In Gram-negative bacteria, Fe3+-siderophore complexes are recognised at the bacterial cell surface by highly selective outer-membrane TonB-dependent transporters (TBDTs). These transporters bind the Fe3+-siderophore complex and translocate it into the periplasm. The structures of pyoverdine, pyochelin, citrate and ferrichrome iron complexes bound to their respective transporters FpvA, FptA, FecA and FhuA showed that the ferric-siderophore complexes were bound inside the barrel adjacent to the plug domain, a position thought to be poised for translocation. Pseudomonas aeruginosa, a serious opportunistic pathogen, does not make enterobactin but does possess a TBTD outer-membrane protein PfeA, related to FepA, that binds and translocates Fe3+-enterobactin into the periplasm. PfeA has the same two domains (22-stranded β-barrel and N-terminal plug) common to the TBDTs.

We constructed four mutants R480A, Q482A, G324V and R480A-Q482A (double mutant) to validate the observed recognition site. Each of the mutant proteins was purified as described for the parent protein, and crystal structures of each were obtained. These structures were essentially identical to that of the parent protein, which confirmed that the mutations did not affect the folding of the protein. Neither G324V nor the double mutant were able to form a complex with Fe3+-enterobactin. The same titration was carried out with G324V and R480A-Q482A, in both these mutants no binding was detected. A R480A-Q482A double mutant and a more radical G324V mutant have the same structure as the native protein, and did not show any detectable binding to Fe3+-enterobactin (ITC experiments, size-exclusion chromatography and crystallography). These results support the genuine nature of the binding site.

> AGQGDGSVIELGEQTVVATAQEETKQAPGVSIITAEDIAKRPPSNDLSQIIRTMPGVNLTGNSSSGQRGNNRQIDIRGMGPENTLILVDGKPVSSRNSVRYGWRGERDSRGDTNWVPADQVERIEVIRGPAAARYGNGAAGGVVNIITKQAGAETHGNLSVYSNFPQHKAEGASERMSFGLNGPLTENLSYRVYGNIAKTDSDDWDINAGHESNRTGKQAGTLPAGREGVRNKDIDGLLSWRLTPEQTLEFEAGFSRQGNIYTGDTQNTNSNNYVKQMLGHETNRMYRETYSVTHRGEWDFGSSLAYLQYEKTRNSRINEGLAVGTEGIFDPNNAGFYTATLRDLTAHGEVNLPLHLGYEQTLTLGSEWTEQKLDDPSSNTQNTEEGGSIPGLAGKNRSSSSSARIFSLFAEDNIELMPGTMLTPGLRWDHHDIVGDNWSPSLNLSHALTERVTLKAGIARAYKAPNLYQLNPDYLLYSRGQGCYGQSTSCYLRGNDGLKAETSVNKELGIEYSHDGLVAGLTYFRNDYKNKIESGLSPVDHASGGKGDYANAAIYQWENVPKAVVEGLEGTLTLPLADGLKWSNNLTYMLQSKNKETGDVLSVTPRYTLNSMLDWQATDDLSLQATVTWYGKQKPKKYDYHGDRVTGSANDQLSPYAIAGLGGTYRLSKNLSLGAGVDNLFDKRLFRAGNAQGVVGIDGAGAATYNEPGRTFYTSLTASF L-glyceraldehyde | C3 H6 O3 | 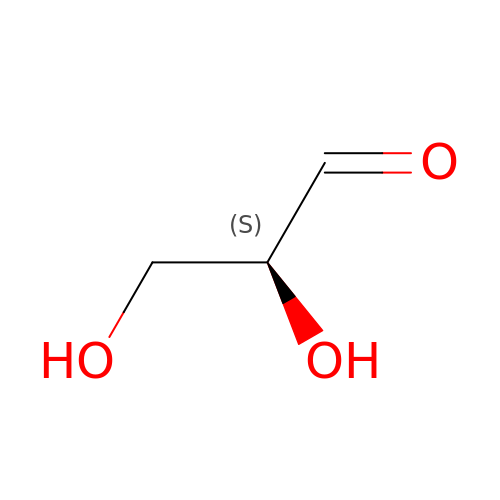MNQZXJOMYWMBOU-GSVOUGTGSA-N To obtain sufficient iron, S. pneumoniae evolved two major highly conserved iron ABC transporters, which are termed Piu (for pneumococcal iron uptake) and Pia (for pneumococcal iron acquisition) systems, respectively. Pia system is responsible for the transport of hydroxamate siderophores such as ferrichrome and ferrioxamin B, whereas Piu system for the transport of heme from hemoglobin. The overall structure of PiaA is composed of an individual N-terminal and a C-terminal domain linked by an α-helix. The N- and C-terminal domains face each other to form a hydrophobic and plastic cleft.

In the complex structure, a molecule of ferrichrome is bound at the center of the inter-domain cleft, with the iron moiety sitting against the bottom of the cleft and the backbone pointing outwards. As shown in the electron density map of the complex structure, the inter-domain cleft captures a molecule of ferrichrome with Λ-cis configuration. The iron moiety of ferrichrome is pulled to the C-terminal domain via three hydrogen bonds with residues Arg231 and Tyr225. In addition, the backbone of ferrichrome is stabilized at the opening side of the inter-domain cleft via three hydrogen bonds with the side chains of Trp158 and Asn83. These six hydrogen bonds keep the ferrichrome to adopt an orientation with the iron moiety pointing inward to the binding cleft. In addition, the methylene carbon atoms of the hydroxyornithine moieties are further packed by a hydrophobic barrel. This barrel is mainly composed of four residues (Met213, Trp223, Tyr225 and Phe255) from the C-terminal domain and three residues (Trp63, Tyr84 and Trp158) from the N-terminal domain. Similar to most class III substrate-binding proteins with a relative rigid linker of α-helix, binding of ferrichrome does not trigger significant conformational changes. Upon ferrichrome binding, the Segments 1 and 2 missing in the apo-form structure undergo significant conformational changes. As a result of induced fit, residues corresponding to the two missing segments are folded into a loop and a η-helix, respectively.

>[2x]MGHHHHHHMNSVKNEENTSKEHAPDKIVLDHAFGQTILDKKPERVATIAWGNHDVALALGIVPVGFSKANYGVSADKGVLPWTEEKIKELNGKANLFDDLDGLNFEAISNSKPDVILAGYSGITKEDYDTLSKIAPVAAYKSKPWQTLWRDMIKIDSKALGMEKEGDELIKNTEARISKELEKHPEIKGKIKGKKVLFTMINAADTSKFWIYTSKDPRANYLTDLGLVFPESLKEFESEDSFAKEISAEEANKINDADVIITYGDDKTLEALQKDPLLGKINAIKNGAVAVIPDNTPLAASCTPTPLSINYTIEEYLNLLGNACKNAK4-({4-[(4-AMINOBUT-2-YNYL)OXY]PHENYL}SULFONYL)-N-HYDROXY-2,2-DIMETHYLTHIOMORPHOLINE-3-CARBOXAMIDE 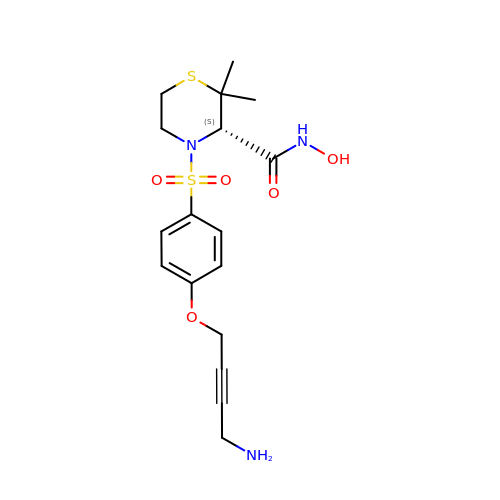| C17 H23 N3 O5 S2 | AANXPIMDONQTQF-HNNXBMFYSA-N>GWNAYIDNLMADGTCQDAAIVGYKDSPSVWA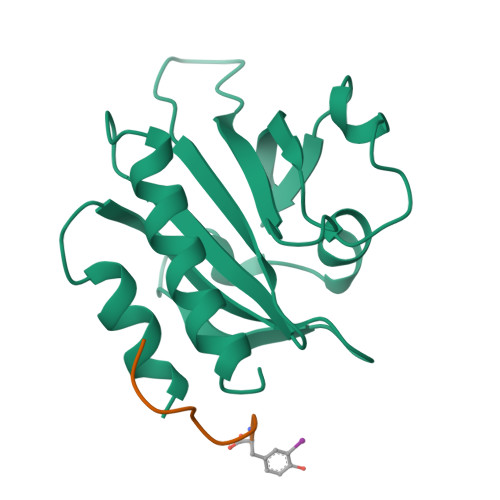AVPGKTFVNITPAEVGVLVGKDRSSFYVNGLTLGGQKCSVIRDSLLQDGEFSMDLRTKSTGGAPTFNVTVTKTDKTLVLLMGKEGVHGGLINKKCYEMASHLRRSQY[2x];> PPPPPPPPY>MKIRKYMRINYYIILKVLVINGSRLEKKRLRSEILKRFDIDISDGVLYPLIDSLIDDKILREEEAP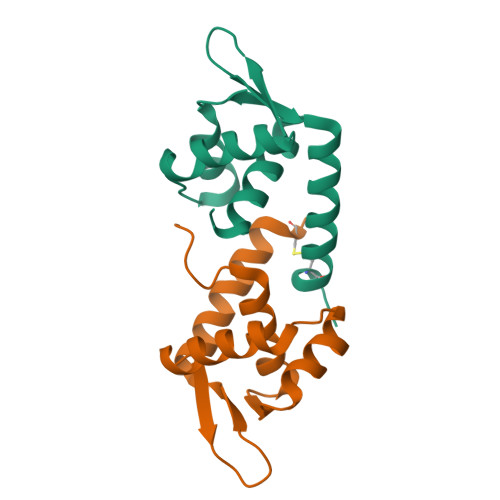DGKVLFLTEKGMKEFEELHEFFKKIVCHHHHHH[2x]> GHMTGVESFMTKQDTTGKIISIDTSSLRAAGRTGWEDLVRKCIYAFFQPQGREPSYARQLFQEVMTRGTASSPSYRFILNDGTMLSAHTR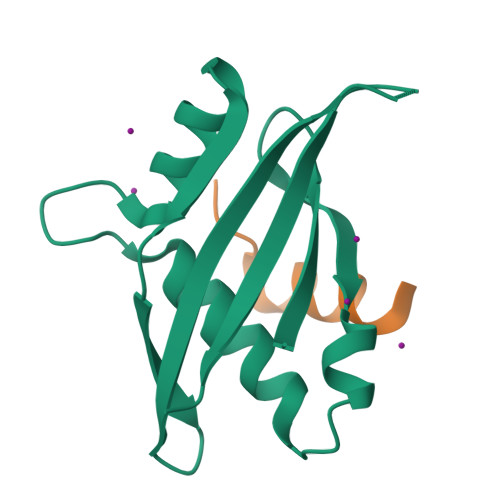CKLCYPQSPDMQPFIMGIHIIDREHSGLSPQDDTNSGMSIPR;> LPPTEQDLTKLLLE> KNNPDPTIYPVLDWNDIKFQDVIGEGNFGQVLKARIKKDGLRMDAAIKRMKEYASKDDHRDFAGELEVLCKLGHHPNIINLLGACEHRGYLYLAIEYAPHGNLLDFLRKSRVLETDPAFAIANSTASTLSSQQLLHFAADVARGMDYLSQKQFIHRDLAARNILVGENYVAKIADFGLSRGQEVYVKKTMGRLPVRWMA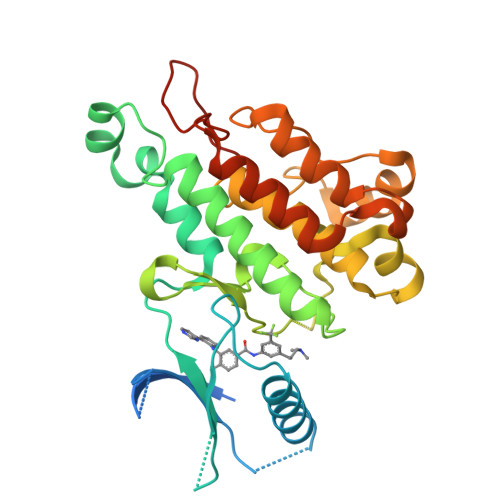IESLNYSVYTTNSDVWSYGVLLWEIVSLGGTPYCGMTCAELYEKLPQGYRLEKPLNCDDEVYDLMRQCWREKPYERPSFAQILVSLNRMLEERKTYVNTTLYEKFTYAGIDCSAEEAA Here, we report the complete structure of a bimodular ∼760 kDa BoNT/A large progenitor toxin complex (L-PTC), which is composed of BoNT and four non-toxic bacterial proteins. We found that L-PTC/A consists of two structurally and functionally independent sub-complexes, the M-PTC and the HA complex. The HA complex is composed of HA70, HA17, and HA33 in a 3∶3∶6 stoichiometry and adopts an extended three-blade architecture, whereas the M-PTC is situated on top of the HA complex platform. BoNT/A absorption is mainly mediated by nine glycan-binding sites on the HA complex that together form multivalent interactions with host carbohydrate receptors on intestinal epithelial cells.

We also determined the crystal structures of the HA17–HA33 complex bound with Gal, Lac, or LacNAc. All three bind to an identical site in HA33, where the HA33–glycan interactions are mediated only by the Gal moiety through extensive hydrogen bonding and a crucial stacking interaction between Phe278 and the hexose ring of Gal. The HA33–Gal interaction is well-defined and identical for the two HA33 molecules in one asymmetric unit (AU). To further confirm the structural findings, we mutated the Gal-binding residues in HA33 (e.g., D263A or F278A) and found that these mutations almost completely abrogated the Lac binding. Gal binds at an equivalent site in HA33 of L-PTC/C (HA33-C) but with ∼15-fold lower binding affinity than with HA33-A, which is likely caused by the replacement of Phe278 in HA33-A with Asp271 in HA33-C. In addition, HA33-C binds Neu5Ac in an adjacent binding site. However, HA33-A does not bind Neu5Ac-containing sugars because the key Neu5Ac-binding residues in HA33-C, Trp176 and Arg183, are replaced in HA33-A with Tyr180 and Asn187, respectively. These differences between HA33-A and HA33-C indicate that the known host susceptibility to different BoNT serotypes may be determined in part by the interaction between HA33 and host glycan receptors.

>[2x]EHYSVIQNSLNDKIVTISCKADTNLFFYQVAGNVSLFQQTRNYLERWRLIYDSNKAAYKIKSMDIHNTNLVLTWNAPTHNISTQQDSNADNQYWLLLKDIGNNSFIIASYKNPNLVLYADTVARNLKLSTLNNSNYIKFIIEDYIISDLNNFTCKISPILDLNKVVQQVDVTNLNVNLYTWDYGRNQKWTIRYNEEKAAYQFFNTILSNGVLTWIFSNGNTVRVSSSNDQNNDAQYWLINPVSDTDETYTITNLRDTTKALDLYGGQTANGTAIQVFNYHGDDNQKWNIRNPPGSA;> GPSVERTFLPNGNYNIKSIFSGSLYLNPVSKSLTFSNESSANNQKWNVEYMAENRCFKISNVAEPNKYLSYDNFGFISLDSLSNRCYWFPIKIAVNTYIMLSLNKVNELDYAWDIYDTNENILSQPLLLLPNFDIYNSNQMFKLEKI>[4x]MSYKSDIEIAQEAKIEHIKDVATKIGLCEDDIEYYGKYKAKIDYNLLKRFEDKKDAKLILTTAINPTPAGEGKTTTTVGLGDALRRLGKNAMIALREPSLGPVFGIKGGAAGGGYAQVVPMEDINLHFTGDFHAIGAANNLL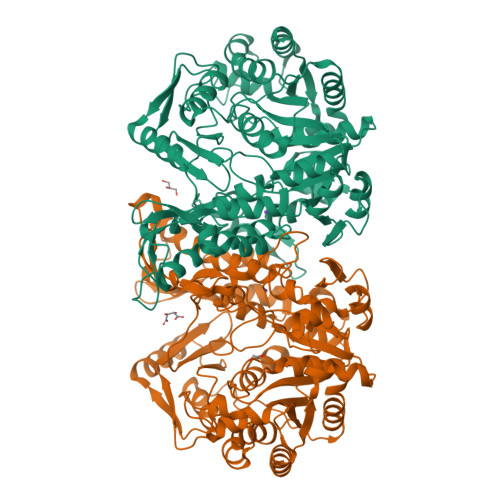AAMIDNHIYQGNELNIDPRRITWKRCVDMNDRQLRFVVDGLGGKANGTPREDGYDITVASEIMAVFCLANDMEDLKNRLARIIIGYTYDGKPVTAGQLKAQGAMAALLKDAFKPNLVQTLEGTPAFVHGGPFANIAHGCNSIIATKMALKLADYVVTEAGFGADLGAEKFLDIKCRMADIRPDAVVIVATIRALKYNGGVKKEDLNQENLDALKKGLPNLLKHVENITEKYGIPTVVAINQFPTDTERELALVQEECNRLGVNAVLSEVWAKGGEGGLELAKEVVRIIEEGKNNFKPIYDLDMGIADKITTIAKEIYGADGVEFAPAALKEINTLEELGFKNVPVCIAKTQYSLTDDPKLLGRPTGFKINVRNVKISAGAGFVVALTGAIMTMPGLPKRPAAEKIDVDVNGKIAGLF9,10-dioxo-4-(phenylamino)-9,10-dihydroanthracene-2-sulfonic acid | C20 H13 N O5 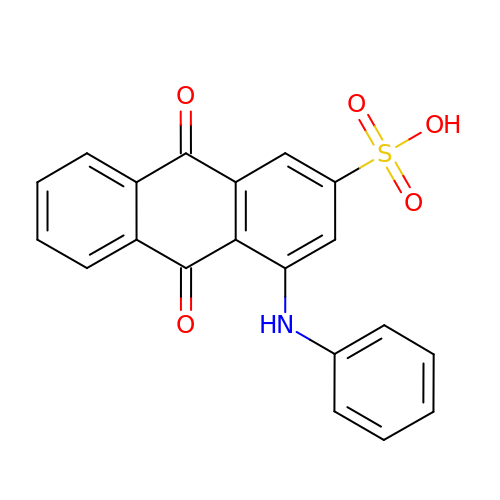S | AAKZMFOUEBXRTE-UHFFFAOYSA-N>MKSVATSSLDDVDKDSVPLGSSINGTAQAETPLENVIDVESVRSHFPVLGGETAAFNNASGTVVLKEAIESTSNFMYSFPFPPGVDAKSMEAITAYTGNKGKVAAFINALPDEITFGQSTTALFRLLGLSLKPMLNNDCEIVCSTLCHEAAASAWIHLSRELGITIKWWSPTTTPNSPDDPVLTTDSLKPLLSPKTRLVTCNHVSNVVGTIHPIREIADVVHTIPGAMLIVDGVASVPHRPVDVKELDVDFYCFSWYKLFGPHLGTLYASRKAQDRYMTSINHYFVSSSSLDGKLALGMPSFELQLMCSPIVSYLQDTVGWDRIVRQETVLVTILLEYLLSKPSVYRVFGRRNSDPSQRVAIVTFEVVGRSSGDVAMRVNTRNRFRITSGTLMAPRPTWDVLKPKSSDGLVRVSFVHYNTVEEVRAFCSELDE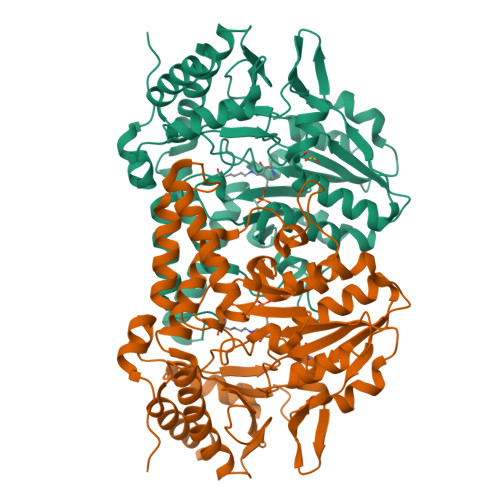IVTRDTLEHHHHHH[3x]[(S)-({2-[hydroxy(methyl)amino]-2-oxoethyl}sulfanyl)(phenyl)methyl]phosphonic acid | C10 H14 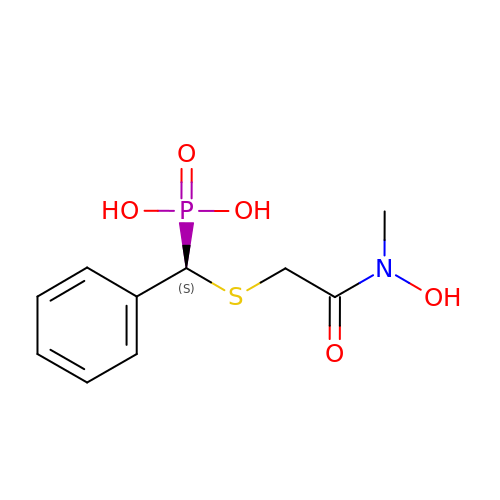N O5 P S | IWQBQVIYTMIQRL-JTQLQIEISA-N>[2x]MRSRRVDVMDVMNRLILAMDLMNRDDALRVTG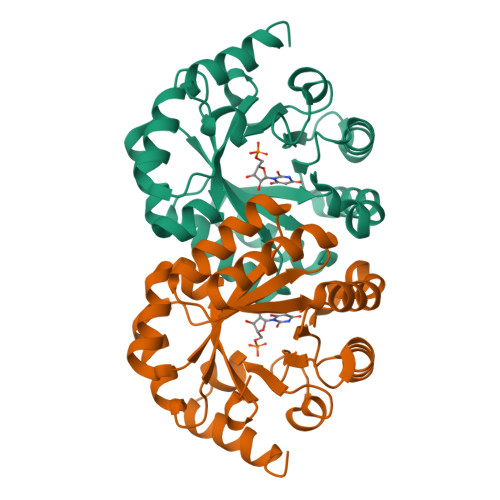EVREYIDTVKIGYPLVLSEGMDIIAEFRKRFGCRIIADFKVADIPETNEKICRATFKAGADAIIVHGFPGADSVRACLNVAEEMGREVFLLTEMSHPGAEMFIQGAADEIARMGVDLGVKNYVGPSTRPERLSRLREIIGQDSFLISPGVGAQGGDPGETLRFADAEIVGRSIYLADNPAAAAAGIIESIKDLLNP> SQDASDGLQRLHMLQISYFRDPYHVWYQGNASLGGHLTHVLEGPDTNTTIIQLQPLQEPESWARTQSGLQSYLLQFHGLVRLVHQERTLAFPLTIRCFLGCELPPEGSRAHVFFEVAVNGSSFVSFRPERALWQADTQVTSG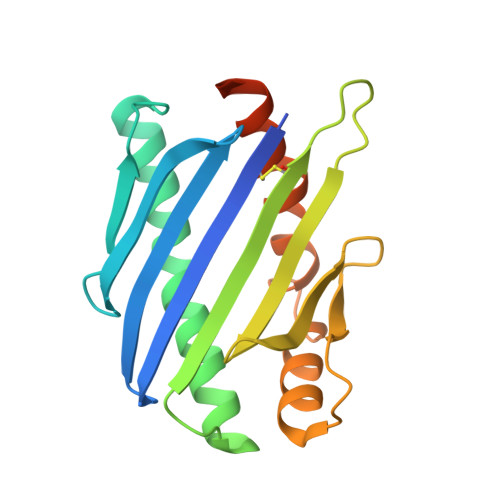VVTFTLQQLNAYNRTRYELREFLEDTCVQYVQKHISAENTKGSQTSRSYTS ADAT2/ADAT3 is a heterodimeric enzyme complex that edits adenosine (A) to inosine (I) at the wobble position 34 of tRNAs starting with an A in their anticodon (ANN-tRNAs). It recognizes specifically tRNAs through the ADAT3 N-terminal domain (ADAT3N), which subsequently rotates to present the bound tRNAs to the ADAT catalytic domain, composed of the C-terminal domain of ADAT3 (ADAT3C) and ADAT2, that carries the catalytic activity. Given the ability of inosine to pair with uracil (U), cytosine (C) or adenosine (A),22 the A to I conversion at position 34 provides an extended base pairing capacity to the modified tRNAs and is essential for decoding the C-ending codons, as GNN-tRNAs do not exist in eukaryotic genomes. Mutations in ADAT3, the catalytically inactive subunit of the ADAT2/ADAT3 complex, have been identified in patients presenting with severe neurodevelopmental disorders.

The ADAT3 V128 residue (corresponding to the V144 residue in humans) is part of a large hydrophobic core located in the middle of the N-terminal domain of ADAT3 (ADAT3N),21 while the ADAT3 A180 residue (corresponding to the A196 residue in humans), is buried within the ADAT3 C-terminal domain (ADAT3C). Crystallization assay of the ADAT2/ADAT3-A180V and ADAT2/ADAT3-A180L complexes were successful for the former complex, while the latter failed to crystallize. Following structure determination at 2.9 Å resolution, comparison with the structure of the WT ADAT2/ADAT3 complex revealed that, unlike the p.V128L variant that mostly affects the ADAT3N, the p.A180V substitution causes small local perturbations in the structure of the ADAT3 C-terminal domain. Here, the crystal structure of the ADAT2/A180V-ADAT3 mutant complex did not reveal any defect in the ADAT3N domain, but rather local perturbations in the α-helix, where the A180 residue is located, and in the ADAT3 C-terminal domain β-sheet, both located close to the interaction surface with ADAT3N. On the other hand, A180 is located in the long α-helix that immediately follows the ADAT3N domain. Co-expressed with ADAT2, the V128M ADAT3 construct was almost as soluble as the WT construct, whereas the A180V and A180L constructs were less soluble, albeit the A180V being slightly more soluble than the A180L construct. While the p.V128M ADAT3 exhibited a significantly impaired enzymatic activity (−68% of A34 to I34 with the lowest concentration of the ADAT2/ADAT3-V128M complex) as expected, the ADAT2/ADAT3-A180V heterodimer retained comparable activity to the WT complex and the ADAT2/ADAT3-A180L displayed a severely diminished deamination capacity (−76% compared with the WT complex at the lowest concentration). Interestingly, the p.A180V variant that does not affect the deamination activity of the ADAT complex as demonstrated in vitro restored the migration defects as efficiently as the ADAT3 WT construct.

> MEEKVESTTTPDGPCVVSVQETEKWMEEAMRMAKEALENIEVPVGCLMVYNNEVVGKGRNEVNQTKNATRHAEMVAIDQVLDWCHQHGQSPSTVFEHTVLYVTVEPCIMCAAALRLMKIPLVVYGCQNERFGGCGSVLNIASADLPNTGRPFQCIPGYRAEEAVELLKTFYKQENPNAPKSKVRKKDCQKS;> GPHMEPTSGFAEQPGPVKAESEEQEPAQWQALPVLSEQQSGAVELILAYAAPVLDKRQTSRLLREVSAVYPLPAQPHLKRVRPSRSAGGAQSSDLLLCLAGPSAGPRSLAELLPRPAVDPRGLGTPFLVPVPARPPLTRSQFEEARAHWPTSFHEDKQVTSALAGQLFSTQERAAMQTHMERVVCAAQRAAAQGLRAVGAVVVDPASDRVLATGHDCSSVASPLLHAVMVCIDLVAQGQGEDSLPYVCTGYDLYVTREPCVMCAMALVHARIQRVFYGAPSPDGALGTLFRVHARPDLNHRFQVFRGILEDQCRQLDPDP3-acetylene 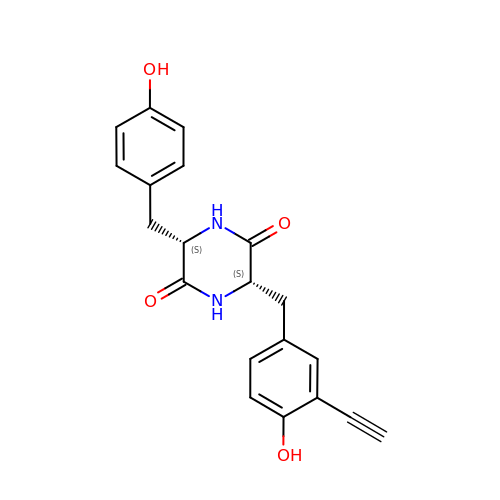dicyclotyrosine | C20 H18 N2 O4 | LIUSUWHATTTWPP-IRXDYDNUSA-N> QGIEDLISEVAQGALTLSLPKQQDSLPDTKASGPAHSKEVPALTAVETGATNPLAPSDTVQTRHVVQRRSRSESTIESFFARGACVAIIEVDNEQPTTRAQKLFAMWRITYKDTVQLRRKLEFFTYSRFDMEFTFVVTANFTNANNGHALNQVYQIMYIPPGAPTPKSWDDYTWQTSSNPSIFYTYGAAPARISVPYVGLANAYSHFYDGFAKVPLKTDANDQIGDSLYSAMTVDDFGVLAVRVVNDHNPTKVTSKVRIYMKPKHVRV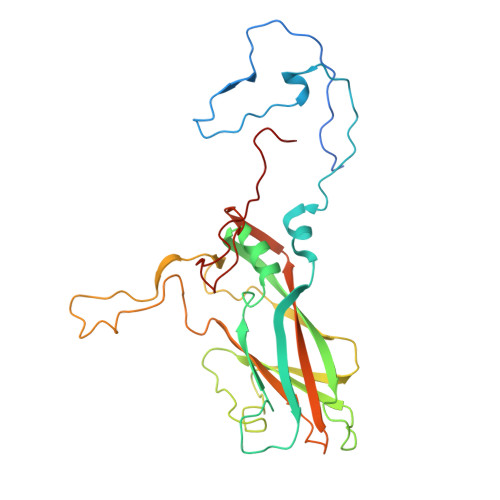WCPRPPRAVPYYGPGVDYRNNLDPLSEKGLTTY> DYKDDDDAMEPSATPGAQMGVPPGSREPSPVPPDYEDEFLRYLWRDYLYPKQYEWVLIAAYVAVFVVALVGNTLVCLAVWRNHHMRTVTNYFIVNLSLADVLVTAICLPASLLVDITESWLFGHALCKVIPYLQAVSVSVAVLTLSFIALDRWYAICHPLLFKSTARRARGSILGIWAVSLAIMVPQAAVMECSSVLPELANRTRLFSVCDERWADDLYPKIYHSCFFIVTYLAPLGLMAMAYFQIFRKLWGRQGIDCSFWNESYLTGSRDERKKSLLSKFGMDEGVTFMFIGRF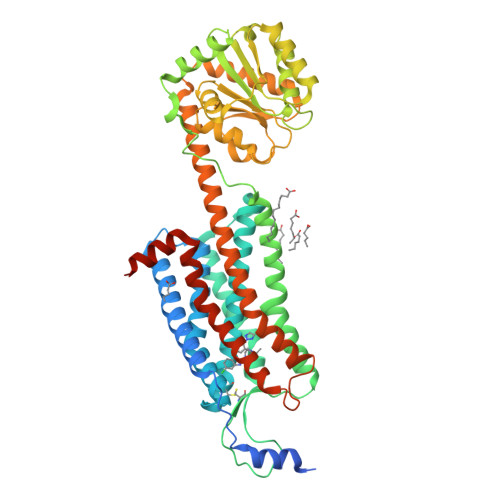DRGQKGVDVLLKAIEILSSKKEFQEMRFIIIGKGDPELEGWARSLEEKHGNVKVITEMLSREFVRELYGSVDFVIIPSYFEPFGLVALEAMCLGAIPIASAVGGLRDIITNETGILVKAGDPGELANAILKALELSRSDLSKFRENCKKRAMSFSKQMRARRKTAKMLMVVLLVFALCYLPISVLNILKRVFGMFRQASDREAVYACFTFSHWLVYANSAANPIIYNFLSGKFREQFKAAFSCCLPGLHHHHHHHHHH>MRGSMIKIIKNAKVFSPEYIGKKDVIFYHKVIHVGEGVNTSVLPFEHEIYDANGLLLLPGLIDPHVHITGGGGEGGFETRTPELKISDCIRSGVTTVVGCLGTDGITRSLENLYAKAKSLESEGLNTFIYTGSYRVPPVTFTGSIMRDIVLIDKVIGVGEIAISDHRSSQPTLEEILRIVADIRVGGMISGKAGIVNFHVGSGKRGIEYLFDIIEKTEIPIQHLYPTHMSRSRKLFEQGLEFAKRGGTIDLTALQPKDAEFVRAEFTTIDAICEAYENGLLDNVTISSDGQGSLPKFDDNGNFVGLDVGSVSAVWYTIRKVLEKGLPLAEVLKISTTNPARVFKLNKGKIAK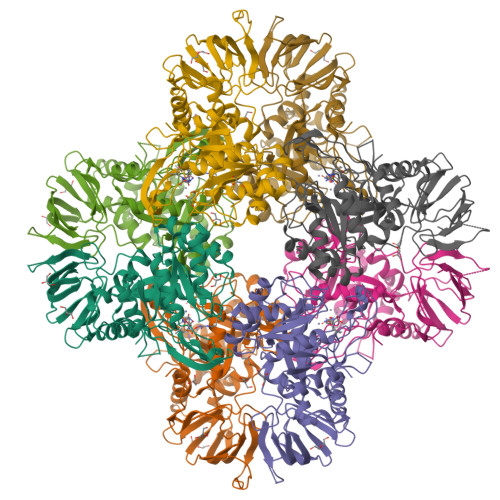GQDADFILVDEQSFEIVSVISKGEFLMKDGVMKNLNFEF[4x]VhCBP is a periplasmic chitooligosaccharide-binding protein mainly responsible for translocation of the chitooligosaccharide (GlcNAc)2 across the double membranes of marine bacteria. The chitooligosaccharide-specific SBP is localized to the periplasmic compartment of the bacterial cell wall and serves as a mobile component of the (GlcNAc)2-specific ABC transporter. SBPs share a common structural feature comprising two domains connected by a flexible hinge region. VcCBP and VhCBP belong to cluster C/subcluster IV (C-IV), members of which are specific for oligosaccharides, including mannooligosaccharides, cellooligosaccharides, and chitooligosaccharides.

The N409A mutation eliminated the hydrogen bond with the reducing-end GlcNAc, but simultaneously, two water molecules fit into the corresponding position. One water molecule interacts with O3 of the reducing-end GlcNAc, whereas the other bridges the N-acetyl carbonyl group and Nη of Arg436. A hydrogen bond of Asn409 with O3 of the GlcNAc at site 2 is eliminated by the N409A mutation; however, two water molecules were introduced into the VhCBP–(GlcNAc)2 interface. This may be the cause of the decreased enthalpic term and increased entropic term listed in Table 3. Finally, the N409A mutation resulted in a small decrease in the binding affinity.

> AERSELTIHPKEFTTFVRNFNPFLGATNLHTTTDFIYEPLVVFNEMHGNTPVFRLAENFQMSDDLMSVTFDIRKGVKWSDGEAFTADDVVYSFNLVKEKPELDQSGINSWVTGVEKVNDYQVKFRLSEANSNVPYEIAKVPVVPKHVWSKVKDPSTFTNENPVGSGPFTVIDTFTPQLYIQCENPNYWDAANLDVDCLRVPQIANNDQFLGKVVNGEMDWTSSFVPDIDRTYAAASPKHHYWYPPAGTQAFVVNFKNPDAAKNEALTNVDFRRAFSMALDRQTIIDIAFYGGGTVNDFASGLGYAFEAWSDEKTHDKFKAYNSYNAEGAKKLLAKAGFKDVNKDGFVDTPSGKSFELLIQSPNGWTDFNNTVQLAVEQLAEVGIKARARTPDFSVYNQAMLEGTYDVAYTAYFHGADPYTYWNSAYNSALQSGDGMPRFAMHFYKNEKLDGLLNSFYKTADKQEQLEIAHGIQQIIAQDQVTIPVLSGAYMYQYNTTRFTGWWNEENPKGRPNIWAGIPERLLHVLDLKPVKHHHHHH Endoxifen | C25 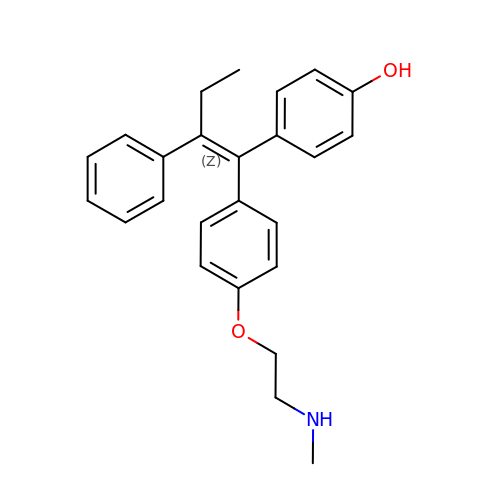H27 N O2 | MHJBZVSGOZTKRH-IZHYLOQSSA-N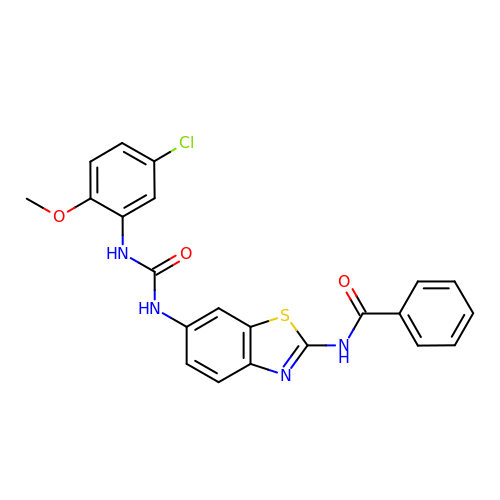N-(6-{[(5-chloro-2-methoxyphenyl)carbamoyl]amino}-1,3-benzothiazol-2-yl)benzamide | C22 H17 Cl N4 O3 S | GFYCKNKAOMHFQF-UHFFFAOYSA-N> MGSSHHHHHHSQDPNSMTTLTRQDLNFGQVVADVLCEFLEVAVHLILYVREVYPVGIFQKRKKYNVPVQMSCHPELNQYIQDTLHCVKPLLEKNDVEKVVVVILDKEHRPVEKFVFEITQPPLLSISSDSLLSHVEQLLAAFILKISVCDAVLDHNPPGCTFTVLVHTREAATRNMEKIQVIKDFPWILADEQDVHM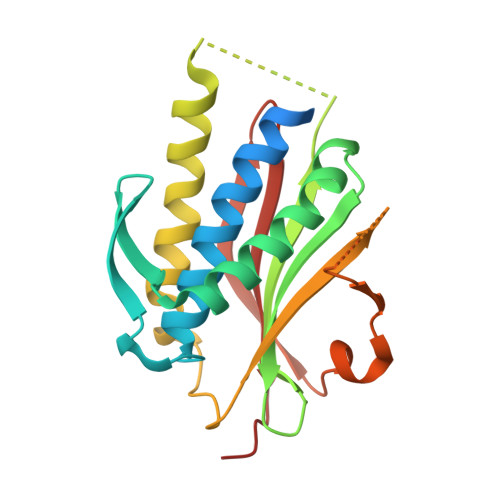HDPRLIPLKTMTSDILKMQLYVEERAHKGS>[3x]MATPSMMPQWSYMHISGQDASEYLSPGLVQFARATETYFSLNNKFRNPTVAPTHDVTTDRSQRLTLRFIPVDREDTAYSYKARFTLAVGDNRVLDMASTYFDIRGVLDRGPT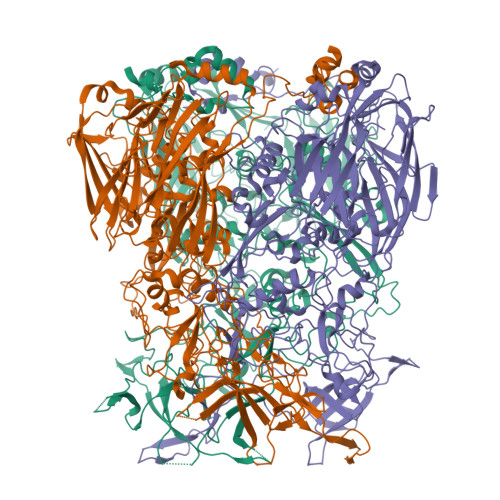FKPYSGTAYNALAPKGAPNPCEWDEAATALEINLEEEDDDNEDEVDEQAEQQKTHVFGQAPYSGINITKEGIQIGVEGQTPKYADKTFQPEPQIGESQWYETEINHAAGRVLKKTTPMKPCYGSYAKPTNENGGQGILVKQQNGKLESQVEMQFFSTTEATAGNGDNLTPKVVLYSEDVDIETPDTHISYMPTIKEGNSRELMGQQSMPNRPNYIAFRDNFIGLMYYNSTGNMGVLAGQASQLNAVVDLQDRNTELSYQLLLDSIGDRTRYFSMWNQAVDSYDPDVRIIENHGTEDELPNYCFPLGGVINTETLTKVKPKTGQENGWEKDATEFSDKNEIRVGNNFAMEINLNANLWRNFLYSNIALYLPDKLKYSPSNVKISDNPNTYDYMNKRVVAPGLVDCYINLGARWSLDYMDNVNPFNHHRNAGLRYRSMLLGNGRYVPFHIQVPQKFFAIKNLLLLPGSYTYEWNFRKDVNMVLQSSLGNDLRVDGASIKFDSICLYATFFPMAHNTASTLEAMLRNDTNDQSFNDYLSAANMLYPIPANATNVPISIPSRNWAAFRGWAFTRLKTKETPSLGSGYDPYYTYSGSIPYLDGTFYLNHTFKKVAITFDSSVSWPGNDRLLTPNEFEIKRSVDGEGYNVAQCNMTKDWFLVQMLANYNIGYQGFYIPESYKDRMYSFFRNFQPMSRQVVDDTKYKDYQQVGILHQHNNSGFVGYLAPTMREGQAYPANFPYPLIGKTAVDSITQKKFLCDRTLWRIPFSSNFMSMGALTDLGQNLLYANSAHALDMTFEVDPMDEPTLLYVLFEVFDVVRVHRPHRGVIETVYLRTPFSAGNATT> MKKQNDIPQPIRGDKGATVKIPRNIERDRQNPDMLVPPETDHGTVSNMKFSFSDTHNRLEKGGYAREVTVRELPISENLASVNMRLKPGAIRELHWHKEAEWAYMIYGSARVTIVDEKGRSFIDDVGEGDLWYFPSGLPHSIQALEEGAEFLLVFDDGSFSANSTFQLTDWLAHTPKEVIAANFGVTKEEISNLPGKEKYIFENQLPGSLKDDIVEGPNGEVPYPFTYRLLEQEPIESEGGKVYIADSTNFKVSKTIASALVTVEPGAMRELHWHPNTHEWQYYISGKARMTVFASDGHARTFNYQAGDVGYVPFAMGHYVENIGDEPLVFLEIFKDDHYADVS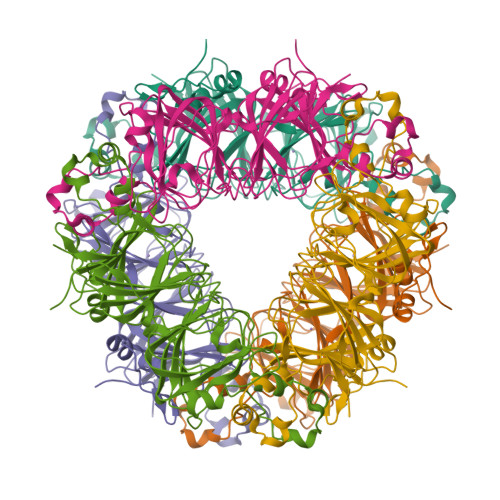LNQWLAMLPETFVQAHLDLGKDFTDVLSKEKHPVVKKKCSK> MSTPSVHCLKPSPLHLPSGIPGSPGRQRRHTLPANEFRCLTPEDAAGVFEIEREAFISVSGNCP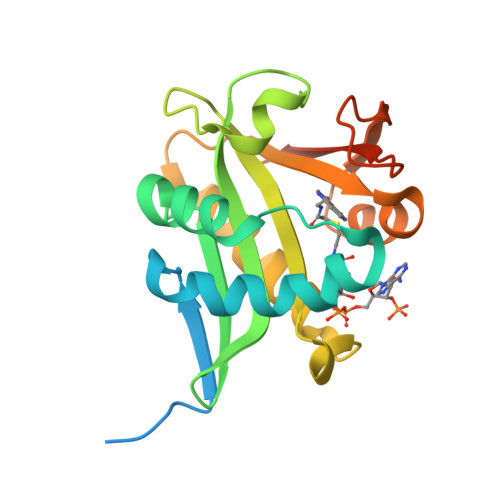LNLDEVQHFLTLCPELSLGWFVEGRLVAFIIGSLWDEERLTQESLALHRPRGHSAHLHALAVHRSFRQQGKGSVLLWRYLHHVGAQPAVRRAVLMCEDALVPFFQRFGFHPAGPCAIVVGSLTFTEMHCSLRGHAALRRNSDR> LV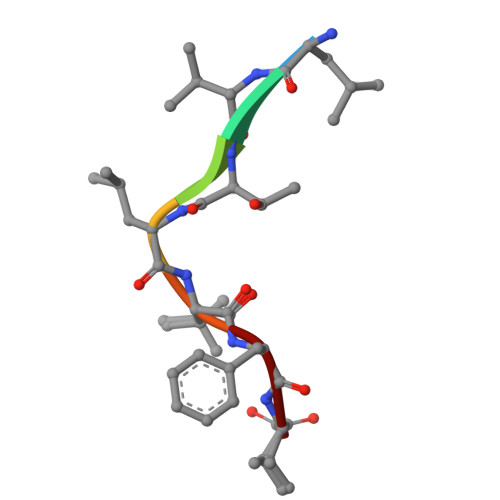TLVFV1-methyl-4-{[3-(2-oxopropyl)-1,3-benzothiazol-3-ium-2-yl]methyl}quinolin-1-ium 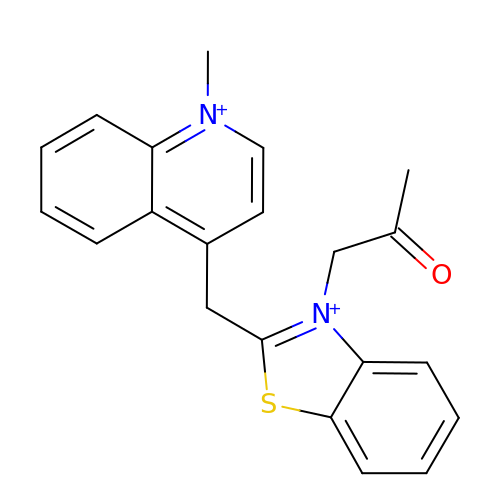| C21 H20 N2 O S | HTPXDOYVWJQKFJ-UHFFFAOYSA-N> APVRSLNCTLRDSQQKSLVMSGPYELKALHLQGQDMEQQVVFSMSFVQGEESNDKIPVALGLKEKNLYLSCVLKDDKPTL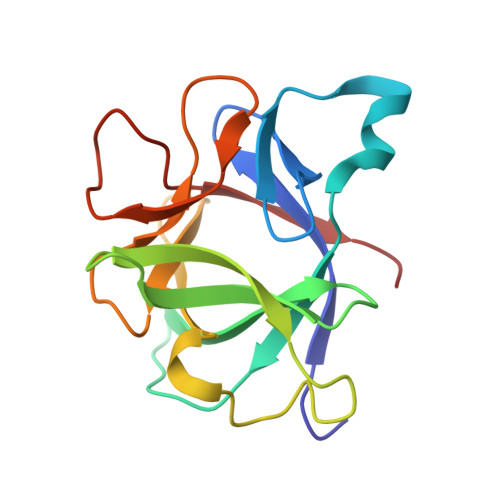QLESVDPKNYPKKKMEKRFVYNKIEINNKLEFESAQFPNWYISTSQAENMPVFLGGTKGGQDITDFTMQFVSS>[2x]AVEQCDLSQFQTTSSNQLMAAIRQQGASCVNALFSADTGVQEAAFSSNHMYNVAQYTRTLAQQYAGGGSDELEALYLYLRAGYYAEFYNSNITFLSWVTPAVKGAVDAFVQNAHFYDNGDAHGKVLNEVIITMDSAGLQHAYLDVVTQWLTRWNAQYAEHWYMRNAVNGVFTLLFGGQWNNQYTSLIGEQTALVTALQAFALDRTKVNSPTEFMAANAARELGRLARYTDATIAPKVTEGLTAIFGQYPSYGDGDAIWLGAA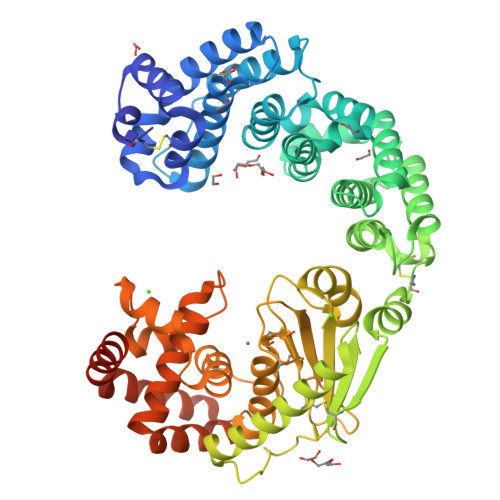DTASYYADCSQFNICGFEDALRDAALNQTFICSDTIKIRSQDMSQAQHLAACDKMAYEESFFHTTLETGNQPVADDHNTQLQVNIFNSDTDYGKYAGPIFGIDTNNGGMYLEGNPANVGNIPNFIAYEASYANPDHFVWNLEHEYVHYLDGRFNMYGDFGTPTELVVWWSEGVAEYVSRVNDNPQAIATIQDGSTYTLAQVFDTTYDGFDVDRIYRWGYLAVRFMFERHPDEVQRMLSATRQGRWAEYKAIISGWANQYQSEFAQWTEALAKGDSGAGNGEGTGSGNEGGGESGGNT> MSVVTTRARIAET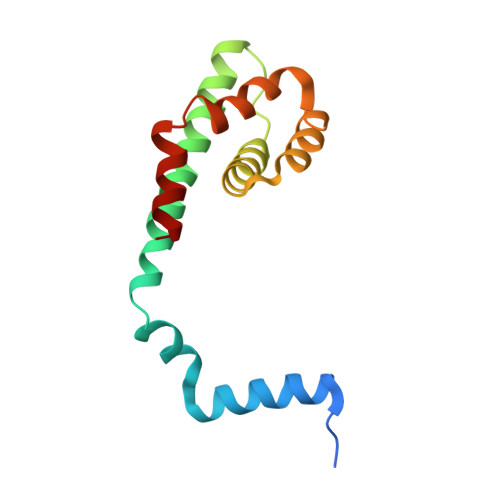LTEKHTLGIEKVVATDSWRVGITSREKKLERINISAEISRRIQDEAIAYARNKGIPYLPGINGIAWKLLRLKWLGYTDQINVVMRTVPAEWRDFLTQIMENTQMESMYSELRKVRV>MGPVWRKHYITYRINNYTPDMNREDVDYAIRKAFQVWSNVTPLKFSKINTGMADILVVFARGAHGDDHAFDGKGGILAHAFGPGSGIGGDAHFDEDEFWTTHSGGTNLFLT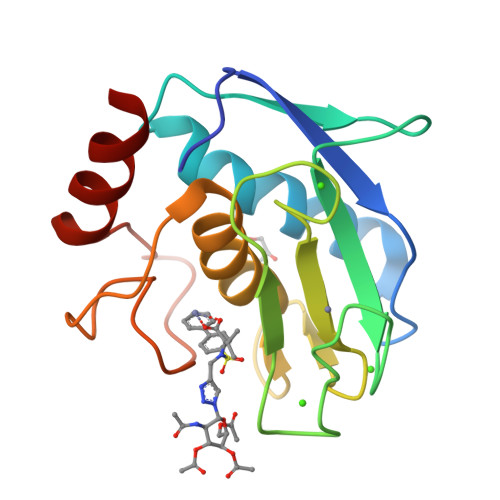AVHQIGHSLGLGHSSDPKAVMFPTYKYVDINTFRLSADDIRGIQSLYG[4x]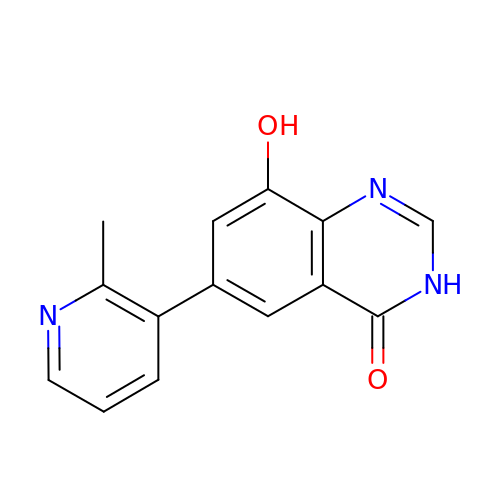6-(2-methylpyridin-3-yl)-8-oxidanyl-3~{H}-quinazolin-4-one | C14 H11 N3 O2 | VPSVVKQCDRXIFW-UHFFFAOYSA-N>MKILVTGAAGFIGSHLCQALLKNSAYHVVGIDHFIGPTPATLKTGNIQSLELNSRFQFIREDILNTDLSKLLQDIDVVYHLAAIPGVRTSWGKDFQPYVTNNIMVTQQLLEACKHIKLDKFIHISTSSVYGEKSGAVSEDLLPIPLSPYGVTKLSGEHLCHVYHKNFHIPIVILRYFTVYGPRQRPDMAFHRLIKQMLEDKPLTIFGDGTQTRDFTYIDDCIR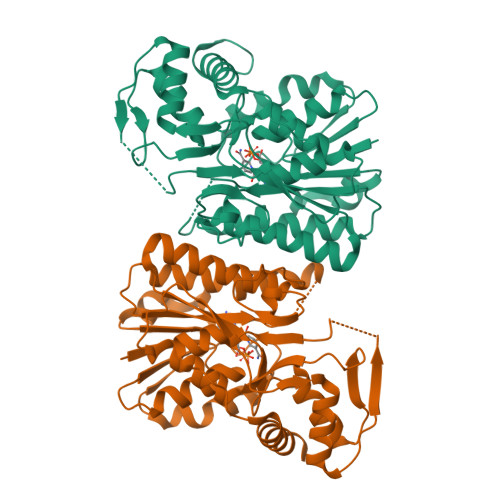GTVAALETKKNIIGEVINIGGKEQASILDIISMLEKISGKSATKNFLKSVPGEPKQTWADISKASTLLQYSPTVSLSDGLEAEYDYIKQLYKGDAAWSHPQFEK[4x]>[2x]MHHHHHHLVPRGSMLDFEKPLFEIRNKIESLKESQDKNDVDLQEEIDMLEASLERETKKIYTNLKPWDRVQIARLQERPTTLDYIPYIFDSFMELHGDRNFRDDPAMIGGIGFLNGRAVTVIGQQRGKDTKDNIYRNFGMAHPEGYRKALRLMKQAEKFNRPIFTFIDTKGAYPGKAAEERGQSESIATNLIEMASLKVPVIAIVIGEGGSGGALGIGIANKVLMLENSTYSVISPEGAAALLWKDSNLAKIAAETMKITAHDIKQLG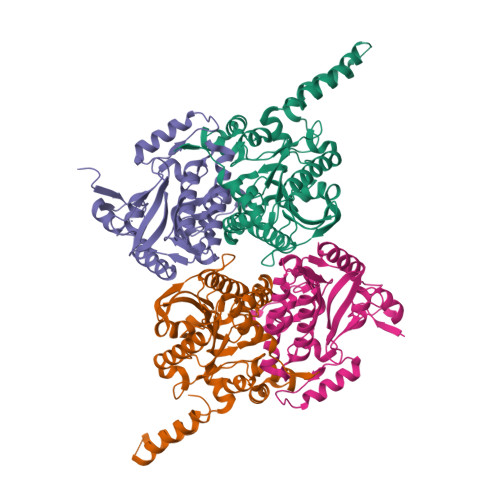IIDDVISEPLGGAHKDIEQQALAIKSAFVAQLDSLESLSRDEIANDRFEKFRNIGSYIE;>[2x]MFKDFFNRTKKKKYLTVQDSKNNDVPAGIMTKCPKCKKIMYTKELAENLNVCFNCDHHIALTAYKRIEAISDEGSFTEFDKGMTSANPLDFPSYLEKIEKDQQKTGLKEAVVTGTAQLDGMKFGVAVMDSRFRMGSMGSVIGEKICRIIDYCTENRLPFILFSASGGARMQEGIISLMQMGKTSVSLKRHSDAGLLYISYLTHPTTGGVSASFASVGDINLSEPKALIGFAGRRVIEQTINEKLPDDFQTAEFLLEHGQLDKVVHRNDMRQTLSEILKIHQEVTK>KKRVFTFGKGRSEGNRDMKSLLGGKGANLAEMSSIGLSVPPGLTISTEACEEYQQNGKSLPPGLWDEISEGLDYVQKEMSASLGDPSKPLLLSVRSGAAISMPGMMDTVLNLGLNDEVVAGLAGKSGARFAYDSYRRFLDMFGNVVMGIPHSLFDEKLEQMKAEKGIHLDTDLTAADLKDLVEKYKNVYVEAKGEKFPTDPKKQLELAVNAVFDSWDSPRANKYRSINQITGLKGTAVNIQSMVFGNMGNTSGTGVLFTRNPSTGEKKLYGEFLINAQGEDVVAGIRTPEDLGTME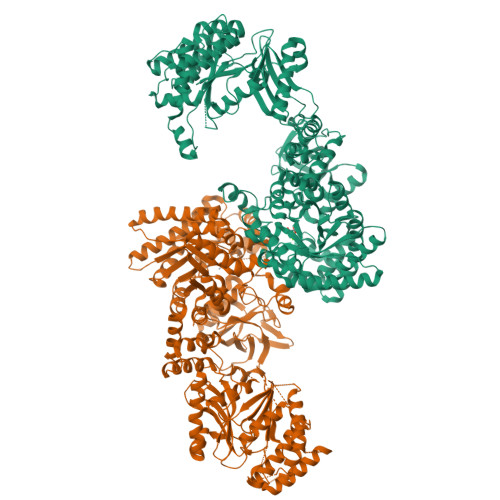TCMPEAYKELVENCEILERHYKDMMDIEFTVQENRLWMLQCRTGKRTGKGAVRIAVDMVNEGLIDTRTAIKRVETQHLDQLLHPQFEDPSAYKSHVVATGLPASPGAAVGQVCFSAEDAETWHAQGKSAILVRTETSPEDVGGMHAAAGILTARGGMTSHAAVVARGWGKCCVSGCADIRVNDDMKIFTIGDRVIKEGDWLSLNGTTGEVILGKQLLAPPAMSNDLEIFMSWADQARRLKVMANADTPNDALTARNNGAQGIGLCRTEHMFFASDERIKAVRKMIMAVTPEQRKVALDLLLPYQRSDFEGIFRAMDGLPVTIRLLDPPLHEFLPEGDLEHIVNELAVDTGMSADEIYSKIENLSEVNPMLGFRGCRLGISYPELTEMQVRAIFQAAVSMTNQGVTVIPEIMVPLVGTPQELRHQISVIRGVAANVFAEMGVTLEYKVGTMIEIPRAALIAEEIGKEADFFSFGTNDLTQMTFGYSRDDVGKFLQIYLAQGILQHDPFEVIDQKGVGQLIKMATEKGRAANPSLKVGICGEHGGEPSSVAFFDGVGLDYVSCSPFRVPIARLAAAQVIV[2x]>[4x]MSRVSTAPSGKPTAAHALLSRLRDHGVGKVFGVVGREAASILFDEVEGIDFVLTRHEFTAGVAADVLARITGRPQACWATLGPGMTNLSTGIATSVLDRSPVIALAAQSESHDIFPNDTHQCLDSVAIVAPMSKYAVELQRPHEITDLVDSAVNAAMTEPVGPSFISLPVDLLGSSEGIDTTVPNPPANTPAKPVGVVADGWQKAADQAAALLAEAKHPVLVVGAAAIRSGAVPAIRALAERLNIPVITTYIAKGVLPVGHELNYGAVTGYMDGILNFPALQTMFAPVDLVLTVGYDYAEDLRPSMWQKGIEKKTVRISPTVNPIPRVYRPDVDVVTDVLAFVEHFETATASFGAKQRHDIEPLRARIAEFLADPETYEDGMRVHQVIDSMNTVM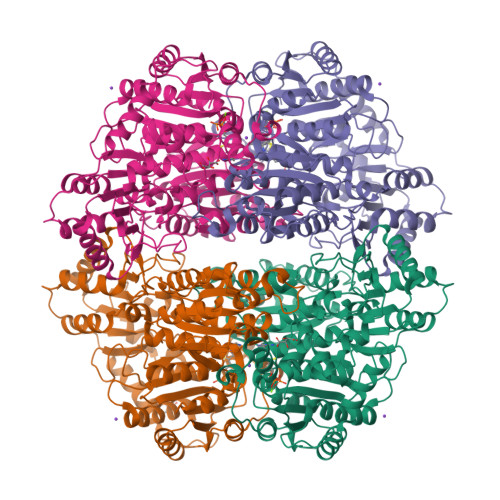EEAAEPGEGTIVSDIGFFRHYGVLFARADQPFGFLTSAGCSSFGYGIPAAIGAQMARPDQPTFLIAGDGGFHSNSSDLETIARLNLPIVTVVVNNDTNGLIELYQNIGHHRSHDPAVKFGGVDFVALAEANGVDATRATNREELLAALRKGAELGRPFLIEVPVNYDFQPGGFGALSI> RETHFLKIPIGDLNIITQDNMKSCQMTTPVIDVIQMLTQGRVSSVPIIDENGYLINVYEAYDVLGLIKGGIYNDLSLSVGEALMR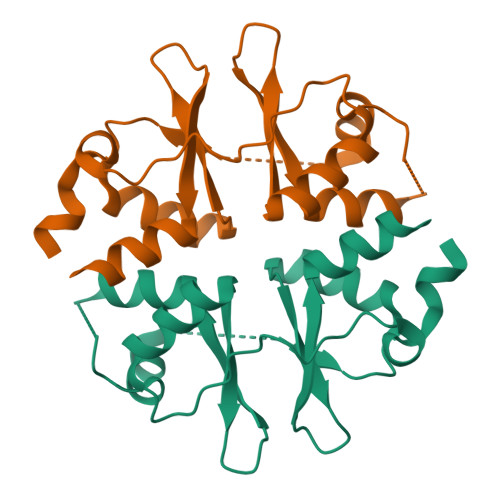RSDDFEGVYTCTKNDKLSTIMDNIRKARVHRFFVVDDVGRLVGVLTLSDILKYILLGSN> ATAAEIAALPRQKVELVDPPFVHAHSQVAEGGPKVVEFTMVIEEKKIVIDDAGTEVHA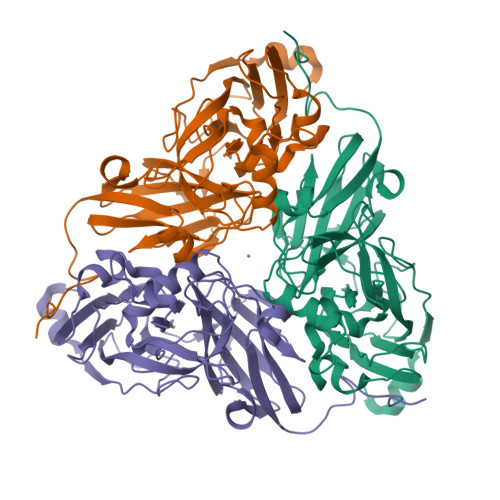MAFNGTVPGPLMVVHQDDYLELTLINPETNTLMHNINFHAATGALGGGGLTEINPGEKTILRFKATKPGVFVYHCAPPGMVPWHVVSGMNGAIMVLPREGLHDGKGKALTYDKIYYVGEQDFYVPRDENGKYKKYEAPGDAYEDTVKVMRTLTPTHVVFNGAVGALTGDKAMTAAVGEKVLIVHSQANRDTRPHLIGGHGDYVWATGKFNTPPDVDQETWFIPGGAAGAAFYTFQQPGIYAYVNHNLIEAFELGAAAHFKVTGEWNDDLMTSVLAPSGTIEGR> YFGKLESKLSVIRNLNDQVLFIDQGNRPLFEDMTDSDCRDNAPRTIFIISMYKDSQPRGMAVTISVKCEKISTLSCENKIISFKEMNPPDNIKDTKSDIIFFQRSVPGHDNKMQFESSSYEGYFLACEKERDLFKLILKKEDELGDRSIMFTVQNED;> GPESCTSRPHITV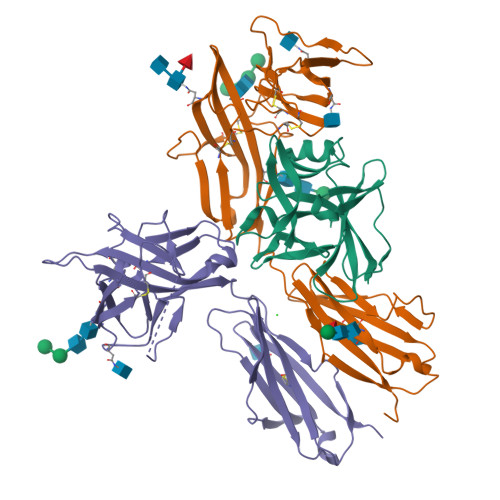VEGEPFYLKHCSCSLAHEIETTTKSWYKSSGSQEHVELNPRSSSRIALHDCVLEFWPVELNDTGSYFFQMKNYTQKWKLNVIRRNKHSCFTERQVTSKIVEVKKFFQITCENSYYQTLVNSTSLYKNCKKLLLENNKNPTIKKNAEFEDQGYYSCVHFLHHNGKLFNITKTFNITIVEDRSNIVPVLLGPKLNHVAVELGKNVRLNCSALLNEEDVIYWMFGEENGSDPNIHEEKEMRIMTPEGKWHASKVLRIENIGESNLNVLYNCTVASTGGTDTKSFILVRKADMADIPGHVFTR;> GPERIKGFNISGCSTKKLLWTYSTRSEEEFVLFCDLPEPQKSHFCHRNRLSPKQVPEHLPFMGSNDLSDVQWYQQPSNGDPLEDIRKSYPHIIQDKCTLHFLTPGVNNSGSYICRPKMIKSPYDVACCVKMILEVKPQTNASCEYSASHKQDLLLGSTGSISCPSLSCQSDAQSPAVTWYKNGKLLSVERSNRIVVDEVYDYHQGTYVCDYTQSDTVSSWTVRAVVQVRTIVGDTKLKPDILDPVEDTLEVELGKPLTISCKARFGFERVFNPVIKWYIKDSDLEWEVSVPEAKSIKSTLKDEIIERNIILEKVTQRDLRRKFVCFVQNSIGNTTQSVQLKEKR>GSNMVKVPECRLADELGGLWENSRFTDCCLCVAGQEFQAHKAILAARSPVFSAMFEHEMEESKKNRVEINDVEPEVFKEMMCFIYTGKAPNLDKMADDLLAAADKYALERLKVMCEDALCSNLSVENAAEILILADLHSADQLKT[2x];>[2x]GSAFPMTMDEKYVNSIWDLLKNAIQEIQRKNNSGLSFEELYRNAYTMVLHKHGEKLYTGLREVVTEHLINKVREDVLNSLNNNFLQTLNQAWNDHQTAMVMIRDILMYMDRVYVQQNNVENVYNLGLIIFRDQVVRYGCIRDHLRQTLLDMIARERKGEVVDRGAIRNACQMLMILGL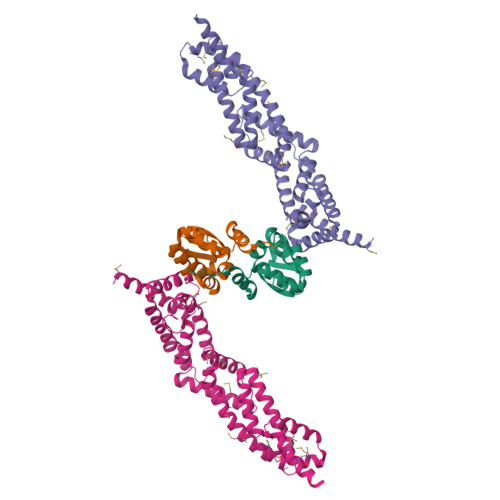EGRSVYEEDFEAPFLEMSAEFFQMESQKFLAENSASVYIKKVEARINEEIERVMHCLDKSTEEPIVKVVERELISKHMKTIVEMENSGLVHMLKNGKTEDLGCMYKLFSRVPNGLKTMCECMSSYLREQGKALVSEEGEGKNPVDYRQGLDDLKSRFDRFLLESFNNDRLFKQTIAGDFEYFLNLN>MERKALVTGGSRGIGRAIAEALVARGYRVAIASRNPEEAAQSLGAVPLPTDLEKDDPKGLVKRALEALGGLHVLVHAAAVNVRKPALELSYEEWRRVLYLHLDVAFLLAQAAAPHMAEAGWGRVLFIGSVTTFTAGGPVPIPAYTTAKTALLGLTRALAKEWARLGIRVNLLCPGYVETEFTLPLRQNPELYEPITARIPMGRWARPEEIARVAAVLCGDEAEYLTGQAVAVDGG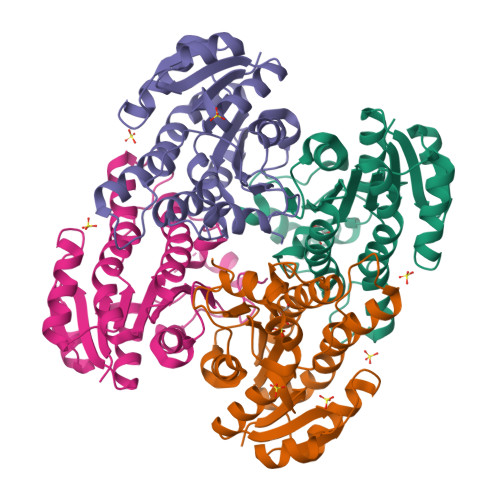FLAY[4x]> KHKILH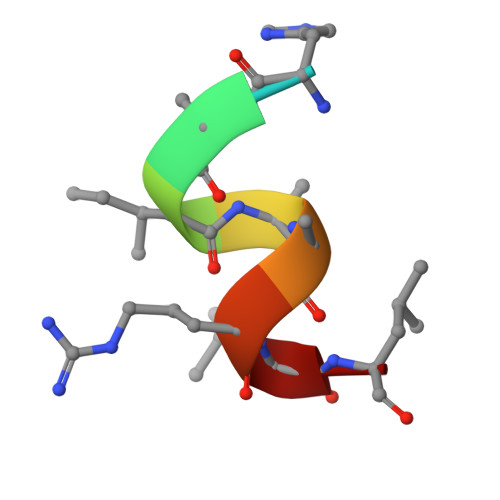RLL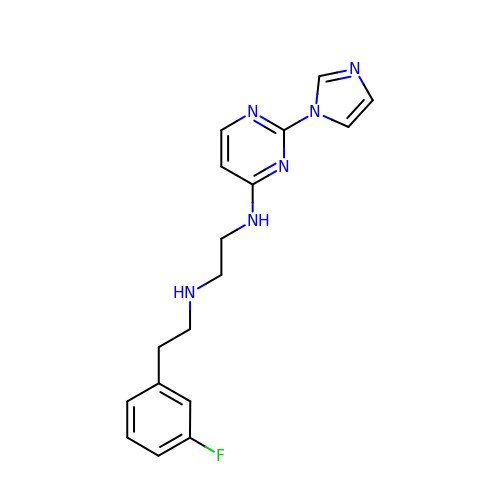N-[2-(3-fluorophenyl)ethyl]-N'-[2-(1H-imidazol-1-yl)pyrimidin-4-yl]ethane-1,2-diamine | C17 H19 F N6 | YCRYBRYYCUMKOD-UHFFFAOYSA-N> MPSPTTVPVATAGRLAEPYIDPAAQVHAIASIIGDVRIAAGVRVAAGVSIRADEGAPFQVGKESILQEGAVIHGLEYGRVLGDDQADYSVWIGQRVAITHKALIHGPAYLGDDCFVGFRSTVFNARVGAGSVIMMHALVQDVEIPPGRYVPSGAIITTQQQADRLPEVRPEDREFARHIIG;> GWLAPEQQQRIYRGNAS

β-Carboxysome biogenesis is reliant on the protein CcmM as a central organizing scaffold. The full-length CcmM protein in Synechococcus elongatus PCC 7942 (Se7942) is a homotrimer of ~58-kDa subunits (SeM58). The N terminus of each M58 protomer consists of a γ-class carbonic anhydrase-like (γCAL) domain that has lost the functional motifs for CA activity, followed by three Rubisco small subunit-like (SSUL) modules connected by flexible linkers. The γCAL domains mediate M58 trimer formation.

To identify the C2 binding site on γCAL, we analyzed the γCAL198–C217 complex by X-ray crystallography. We also solved the structure of γCAL181 in complex with the C217 peptide of CcaA at a resolution of 1.63 Å. The asymmetric unit of the crystal contained the protomer of γCAL181 with one peptide bound. This indicates that all binding sites of the trimeric γCAL181 are occupied by peptide, providing the basis for multivalent network formation between M58 and CcaA. The peptide is bound as a two-turn α-helix (residues PEQQQRIY) in a pocket beneath the protruding β10-β11 loop, making extensive interactions with residues in β11, β17, the β19-β20 loop and α1 of the γCAL protomer. The hydrophobic interactions include π-stacking between the indole ring of residue W257 in the C2 peptide with the benzene ring of F123 (β17) in γCAL. In addition, the hydrophobic residue Y267 of C2 contacts the γCAL residue L81 (β11). Two electrostatic interactions (salt bridges) are formed by the guanidinium group of the peptide residue R265 with E143 (β20) and D163 (α1) of γCAL. Notably, the binding site of C2 is highly conserved in the γCA/γCAL domains of CcmM proteins.>MHAGEAVQQLKKAFETVASFDFRDALSKASTPVTV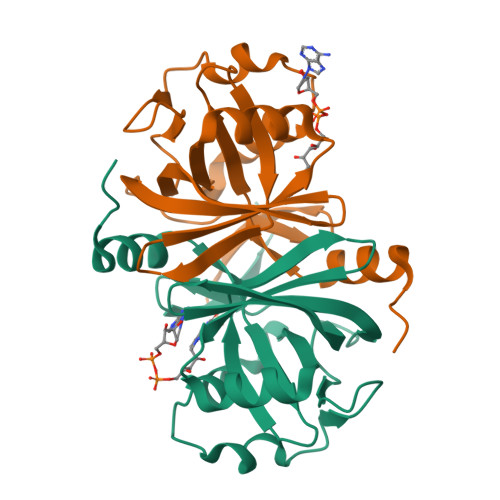VATNGPFGLAGLTCSAVCSVCDRPPTVLLCINRKSYAAGIIKSNGVLSVNWLAAGQAVISQTFAGVGSVPMEERFADKGWQTIATGAPYRMDAAVSFDCTIANIVDVGSHSVIFAEVVARNHAEECTPLIYHRRQYATTRSLAEHHHHHH[2x]>GPMEADGRYYSSKQPYVAPNDATASSYSKAPKGYGPIYTESMA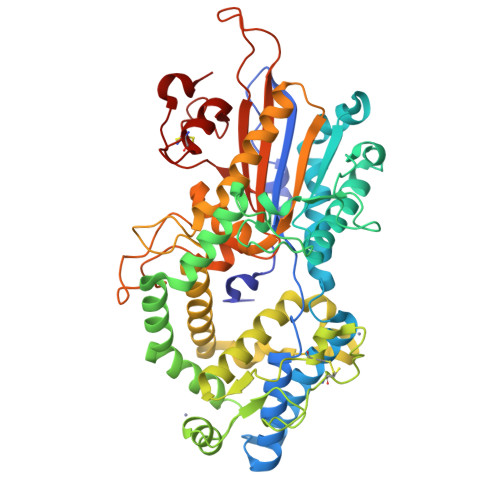RHGSRGLSSYKYDALLMRMAETAARDGGFKSEAIKAEFVKNLSGITAANVENGYGMLTGQGAQQHYGIGERAYQRNRSLFDQAAADGGTIAYQSSGEARATESGENFEKGFNEASGGRLIGNVSAPTNPADSGNGKDFQKNPDTLYFHKVQNPDGTSKVPGTKAYDIANNYQNFVANDATIAGAEKTIGDNVDVKRASHDLLSQIFTEEFLAKLENGEYKWYNTTDGTKKGGKNCAPGADASKDPDACGEVSKKIKSEYDAAMDLYNLYIIAADMHNENTGDHTFAFDQYFQGAYADDARMFAWALDAEDFYEKGPSYAGQNETYSIAQPLLDDFLNTIDARVNGGSTVATFRFAHAETMMPFAALLGLPGSTQQAPASTTDVYTYGNNEWRGESVTPMAANVQWDVYARKGEDPATGQRYTPIVRMLYNENEVPFRSECTPVADGSTWYKLTELKSCLAADHKTLGQDARI[2x]> MGTV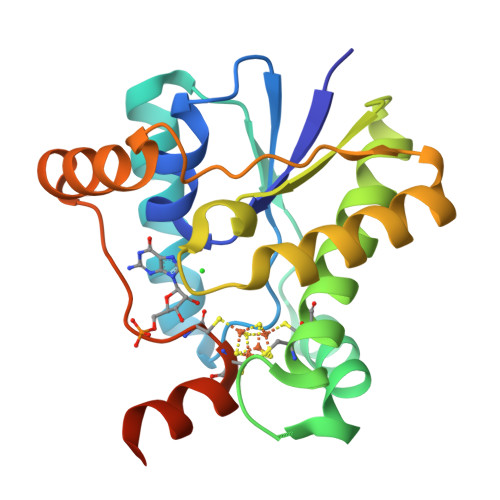LIHVCCAPDLLTTIFHVRDAEFFFYNPNIQPLSEYEKRREAVDKVANHFSLNVRYGEYSTEEIRKWYTAVKDYKDLGEGSKRCERCISFLLERTAQEARKRGHESFSTTLLASPRKNLPMIENIGKTIEEKYGVKFFFKNFRKGGAYQEGVRLSKELGIYRQNYCGCVFSLLERREKHAEISRKRGHM Glutathione transferases (GSTs) are promiscuous enzymes whose main function is the detoxification of electrophilic compounds. The isoenzyme hGSTA1-1 is primarily expressed in the human liver but can also be found in various other human tissues. It is a key enzyme in human physiology, since it is involved in the phase II detoxification mechanism of a wide range of electrophilic compounds, such as drugs, carcinogenic metabolites, and environmental pollutants. Cytosolic GSTs are dimeric enzymes with each subunit having two distinct domains: a conserved N-terminal thioredoxin-like α/β domain and a C-terminal α-helical domain.

The improvement in the catalytic activity of hGSTA1-K141H/S142H as well as its thermal stability prompt us to investigate the structure of this mutant at the atomic level using X-ray crystallography. The mutant was crystallized in two crystal forms with four molecules (1.56 Å resolution) and two molecules (1.87 Å), respectively, in the crystallographic asymmetric unit. The high-resolution structure has Cys112 modified to S,S-(2-hydroxyethyl)thiocysteine, owing to longer storage of the enzyme prior to crystallization. Apart from this, the two structures have only subtle differences, with a root mean square deviation (rmsd) of 0.43 Å. Residues 212–221 at the C-terminal were not included in the structure because of high disorder. The engineered amino acids are at the surface of the enzyme. The results showed that the mutant hGSTA1-K141H/S142H exhibits higher catalytic efficiency, thermal stability, and sensitivity against α-endosulfan compared to the wild-type enzyme. The double mutation K141H/S142H, according to the crystallographic analysis, results in subtle but specific changes in the protein structure, and the observed stability may be attributed to specific interactions within an amino acid network. The results demonstrate that the mutant hGSTA1-K141H/S142H depicts higher catalytic efficiency and stability than the rest of the mutants studied; the mutation S142H is likely the main contributor.

>MAEKPKLHYFNARGRMESTRWLLAAAGVEFEEKFIKSAEDLDKLRNDGYLMFQQVPMVEIDGMKLVQTRAILNYIASKYNLYGKDIKERALIDMYIEGIADLGEMILLLPVCPPEEKDAKLALIKEKIKNRYFPAFEKVLHHHGQDYLVGNKLSRADIHLVELLYYVEELDSSLISSFPLLKALKTRISNLPTVKKFLQPGSPRKPPMDEKSLEEARKIFRF[4x]> MITYVFPGQGSQKQGMGSGLFDEFKELTDQADEILGYSIKRLCLENPYSNLNKTQFTQPALYVVNALSYLKKIRDEEVKPDFVAGHSLGEYNALFAAEAFDFETGLQLVRKRGELMSLISNGGMAAVMGLNEEQVAKALKEYHLHDVDIANVNAPYQIVISGKKDEIEKAASLFETMTEVTMVLPLNVSGAFHSRYMNKAKEEFEEFLHAFYFSPPSIPVISNVYAKPYTYEFMKQTLADQINHSVKWTDSISYLMKKAAMEFEEVGPGNVLTGL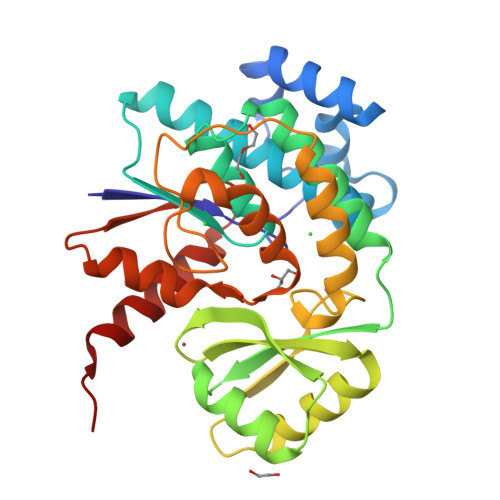IHRIKKDAEAMPR>MKIYIQPLSVNSHTVEVLANSLPKIFNAEVFVLPASDVSLKCYNASRRQYNSTCILRMLPPIKVTLGVTGKDIYAKGMNFVFGEAELGGARAVLSVFRLTTADSELYRERVVKEAVHEIGHVLGLKHCSNNCVMR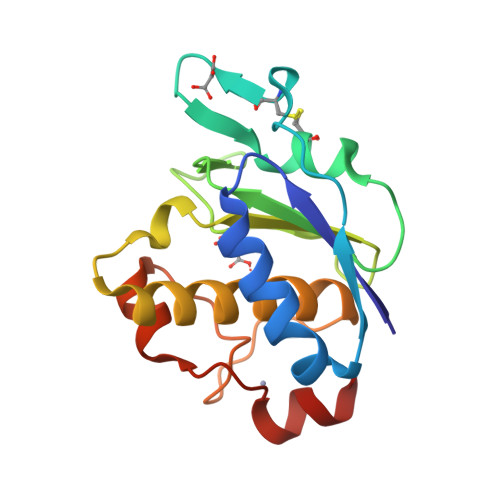FSNSVQDVDRKPVSFCRECASKIRY[3x]> GPMTSQKLVRLPGLIDVHVHLREPGGTHKEDFASGTAAALAGGITMVCAMPNTRPPIIDAPALALAQKLAEAGARCDFALFLGASSENAGTLGTVAGSAAGLKLYLANATTNSSHGVTSVVQWMEHFETWPSHLPIVAHAEQQTVAAVLMVAQLTQRSVHICHVARKEEILLIKAAKARGLPVTCEVAPHHLFLSHDDLERLGPGKGEVRPELGSRQDVEALWENMAVIDCFASDHAPHTLEEKCGSRPPPGFPGLETMLPLLLTAVSEGR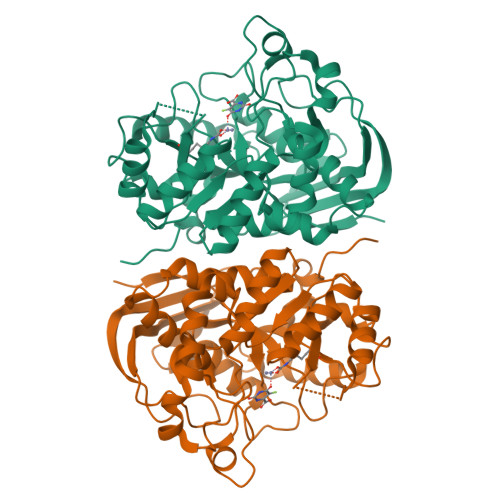LSLDDLLQRLHHNPRRIFHLPPQEDTYVEVDLEHEWTIPSHMPFSKAHWTPFEGQKVKGTVRRVVLRGEVAYIDGQVLVPPGYGQDVRKWPQGAVPQLPPSAPATSEMTTTPERPRRGIPGLPD> SSLGKHNDWIIGKIKYQGNLRTKHMLNPGKVAEQLCREGHRHNVYNKTIGSVMTATGIRLEKLPVVRAQTDTTNFHQAIRDKIDKEENLQTPGLHKKLMEVFNALKRPELESSYDAVEWEELERGINRKGAAGFFERKNIGEILDSEKNKVEEIIDNLKKGRNIKYYETAIPKNEKRDVNDDWTAGDFV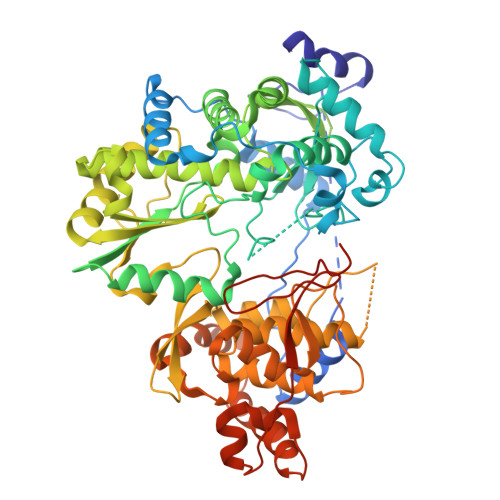DEKKPRVIQYPEAKTRLAITKVMYKWVKQKPVVIPGYEGKTPLFQIFDKVKKEWDQFQNPVAVSFDTKAWDTQVTTKDLELIKDIQKYYFKKKWHKFIDTLTMHMTEVPVICADGEVYIRKGQRGSGQPDTSAGNSMLNVLTMVYAFCEATGVPYKSFDRVAKIHVCGDDGFLITERALGEKFASKGVQILYEAGKPQKITEGDKMKVAYQFDDIEFCSHTPIQVRWSDNTSSYMPGRNTTTILAKMATRLDSSGERGTIAYEKAVAFSFLLMYSWNPLIRRICLLVLSTELQVKPGKSTTYYYEGDPISAYKEVIGHNLFDLKRTSFEKLAKLNLSMSVLGAWTRHTSKRLLQDCVNMGVKEGNWLVNADRLVSSKTGNRYIPGEGHTLQGRHYEELVLARKQINNFQGADRYNGSSSHHHHHH> PAQDNSRFVIRDRNWHPKALTPDYKTSIARSPRQALVSIPQSISETTGPNFSHLGFGAHDHDLLLNFNNGG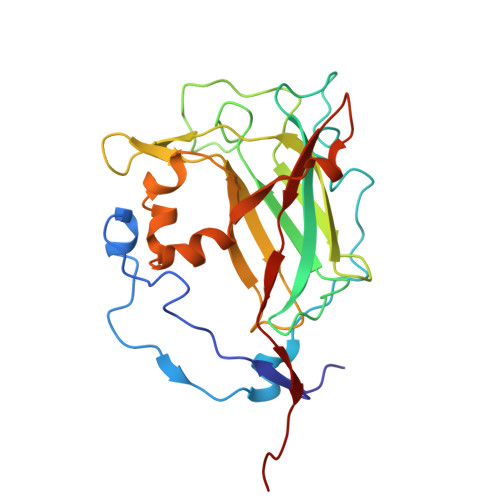LPIGERIIVAGRVVDQYGKPVPNTLVEMWQANAGGRYRHKNDRYLAPLDPNFGGVGRCLTDSDGYYSFRTIKPGPHPWRNGPNDWRPAHIHFGISGPSIATKLITQLYFEGDPLIPMCPIVKSIANPEAVQQLIAKLDMNNANPMDCLAYRFDIVLRGQRKTHFENC>MNNMNVIIADDHPIVLFGIRKSLEQIEWVNVVGEFEDSTALINNLPKLDAHVLITDLSMPGDKYGDGITLIKYIKRHFPSLSIIVLTMNNNPAILSAVLDLDIEGIVLKQGAPTDLPKALAALQKGKKFTPESVSRLLEKISAGGYGDKRLSPKESEVLRLFAEGFLVTEIAKKLNRSIKTISSQKKSAMMKLGVENDIALLNYLSSVTLSPADKD[4x]

At its core are three multidomain proteins, two hybrid histidine kinases (RcsC and RcsD) and a response regulator (RcsB). RcsB belongs to the FixJ/NarL family of response regulators with two domains connected by a long linker. The N-terminal REC (receiver) domain of RcsB is composed of a five-stranded central β-sheet surrounded by five α-helices and contains the conserved aspartyl residue (D56) that serves as the phosphoryl acceptor. The C-terminal DNA-binding domain (helix-turn-helix [HTH]) of RcsB has a four-helix bundle fold with a classical helix-turn-helix DNA recognition motif.

Here, we present crystal structures of unphosphorylated RcsB in complex with the consensus DNA-binding sequence of 22-mer (DNA22) and 18-mer (DNA18) of the flhDC operon from Escherichia coli determined at 3.15- and 3.37-Å resolution, respectively. The asymmetric unit of the RcsB crystal in complex with DNA22 contained one RcsB dimer bound to one double helix DNA, whereas the RcsB crystal in complex with DNA18 contained an RcsB tetramer (two RcsB dimers) bound to two parallel double helical DNAs. In both crystal forms, the RcsB dimers displayed similar structures, and the DNA had a classical B form with an average base pair rise and twist of 3.2 Å and 34°, respectively; the DNA was slightly bent along the surfaces of the RcsB HTH domains. In the structure, the arrangement of the domains of the dimers of RcsB was similar to that of the RcsB dimer found in complex with DNA22. Superposition of dimers in the two structures shows that the average RMSD value was 1.15 Å. Interestingly, within the RcsB tetramer of the RcsB-DNA18 complex, dimers formed asymmetric interfaces between their REC domains. We cannot exclude the existence of a higher-MM RcsB-DNA complex, as indicated by the slowest-migrating band. This putative complex could correspond to an RcsB tetramer bound to two DNAs as seen in our RcsB-DNA18 cocrystal structure. The RcsB-DNA interactions were largely identical at all sites in the structure of RcsB in complex with either DNA22 or DNA18. The structural similarity between RcsB dimers bound to DNA observed in two different crystal forms suggests that this dimer is likely biologically relevant.> MTKMDIRGAVDAAVPTNIIAAKAAEVRANKVNWQSYLQGQMISAED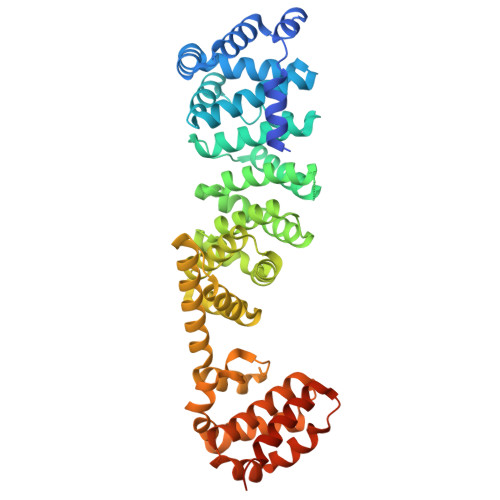CEFIQRFEMKRCSEEKQEMLQTEGSQCAKTFINLMTHISKEQTVQYILTMVDDMLQENHQRVSIFFDYAKRSKSTAWPYFLPMLNRQDPFTVHMAARIIAKLAAWGKELMEGSDLNYYFNWIKTQLSSQKLRGSGVAVETGTISASDSSQYVQCVAGCLQLMLRVNEYRFAWVEADGVNCIMGVLSNKCGFQLQYQMIFSIWLLAFSPQMCEHLRRYNIIPVLSDILQESVKEKVTRIILAAFRNFLEKSTERETRQEYALAMIQCKVLKQLENLEQQKYDDEDISEDIKFLLEKLGESVQDLSSFDEYSSELKSGRLEWSPVHKSEKFWRENAVRLNEKNYELLKILTKLLEVSDDPQVLAVAAHDVGEYVRHYPRGKRVIEQLGGKQLVMNHMHHEDQQVRYNALLAVQKLMVHNWEYLGKQLQSEQPQTAAARS2-{4-[(6-fluoro-1,3-benzothiazol-2-yl)oxy]-2-hydroxyphenyl}-N-methylacetamide | C16 H13 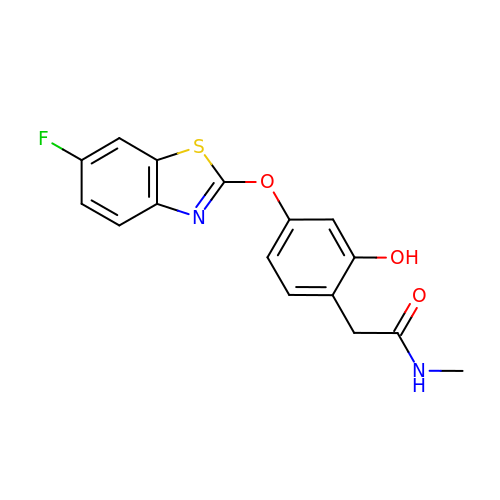F N2 O3 S | VNVALNOVDDOJNH-UHFFFAOYSA-N> MGSNQSSSTSTKKLKAGNFDVAY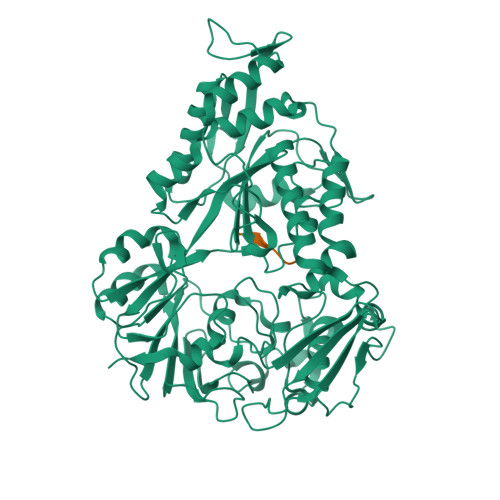QNPDKAIKGGNLKVAYQSDSPMKAQWLSGLSNDATFATMSGPGGGQDGLFFTDSGFKFIKGGAADVALDKESKTATITLRKDLKWSDGSEVTAKDYEFTYETIANPAYGSDRWTDSLANIVGLSDYHTGKAKTISGITFPDGENGKVIKVQFKEMKPGMTQSGNGYFLETVAPYQYLKDVAPKDLASSPKTTTKPLVTGPFKPENVVAGESIKYVPNPYYWGEKPKLNSITYEVVSTAKSVAALSSSKYDIINGMVSSQYKQVKNLKGYKVLGQQAMYISLMYYNLGHYDAKNSINVQDRKTPLQDQNVRQAIGYARNVAEVDNKFSNGLSTPANSLIPPIFKQFTSSSVKGYEKQDLDKANKLLDEDGWKLNKSTGYREKDGKELSLVYAARVGDANAETIAQNYIQQWKKIGVKVSLYNGKLMEFNSWVDHMTTPPGANDWDITDGSWSLASEPSQQDLFSAAAPYNFGHFNDSEITKDLNDIDSAKSENPTYRKAAFVKYQEDMNKKAYVIPTNFMLNYTPVNKRVVGMTLDYGAMNTWSEIGVSSAKLATKGSIEGRHHHHHH;> AASASA>[4x]M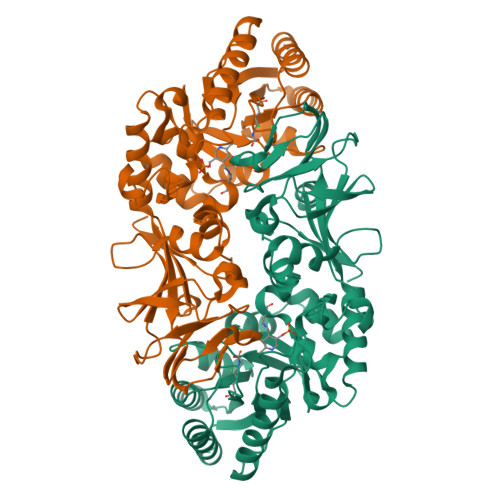GSHHHHHHSSGLVPRGSHMSETTARRDADAVLRARAEIDLAALRANVRALRERAPGAALMAVVKADAYGHGAIPCARAAVAAGATWLGTATPQEALALRAAEPGLPDDVRIMCWLWTPGGPWREAVEARLDVSVSAMWAMEEVTGAARAAGVPARVQLKADTGLGRGGCQPGADWERLVGAALRAEEEGLLRVTGLWSHFACADEPGHPSIAAQLTRFREMTAYAEQRGLRPEVRHIANSPATLTLPDAHFDLVRPGIAMYGVSPSPEIGTPADFGLRPVMTLAASLALVKQVPGGHGVSYGHHYTTPGETTLGLVPLGYADGIPRHASSSGPVLVDGKWRTVAGRIAMDQFVVDLGGDRPEPGAEAVLFGPGDRGEPTAEDWAQAAGTIAYEIVTRIGSRVPRVYVNE[[(2R,3S,4R,5R)-5-(5-aminocarbonyl-3,4-dihydro-2H-pyridin-1-yl)-3,4-bis(oxidanyl)oxolan-2-yl]methoxy-oxidanyl-phosphoryl] 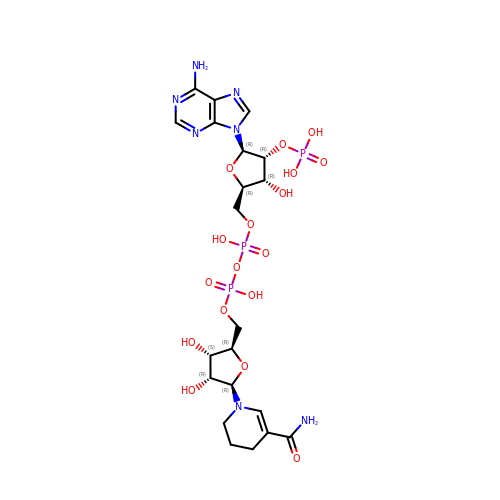[(2R,3R,4R,5R)-5-(6-aminopurin-9-yl)-3-oxidanyl-4-phosphonooxy-oxolan-2-yl]methyl hydrogen phosphate | C21 H32 N7 O17 P3 | XBYZUJOLVDCGQT-NNYOXOHSSA-N>MSPILGYWKIKGLVQPTRLLLEYLEEKYEEHLYERDEGDKWRNKKFELGLEFPNLPYYIDGDVKLTQSMAIIRYIADKHNMLGGCPKERAEISMLEGAVLDIRYGVSRIAYSKDFETLKVDFLSKLPEMLKMFEDRLCHKTYLNGDHVTHPDFMLYDALDVVLYMDPMCLDAFPKLVCFKKRIEAIPQIDKYLKSSKYIAWPLQGWQATFGGGDHPPKSDLEVLFQGPLGSMALVPVGMAPRQMRVNRCIFASIVSFDACITYKSPCSPDAYHDDGWFICNNHLIKRFKMSKMVLPIFDEDDNQFKMTIARHLVGNKERGIKRILIPSATNYQDVFNLNSMMQAEQLIFHLIYNNENAVNTICDNLKYTEGFTSNTQRVIHSVYATTKSILDTTNPNTFCSRVSADELRFFDVTNARALRGGAGDQLFNNYSGFLQN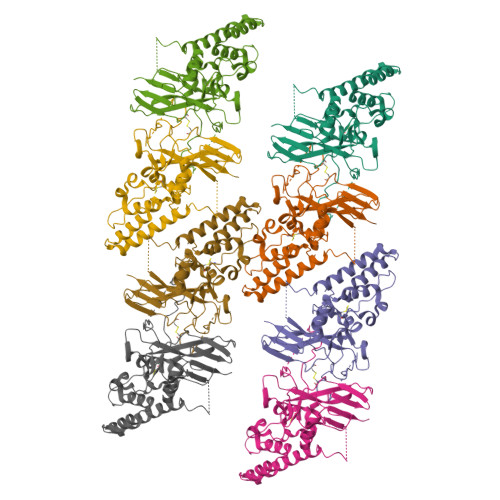LIRRAVAPEYLQIDTEELRFRNCATCIIDETGLVASVPDGPELYNPIRSSDIMRSQPNRLQIRNVLKFEGDTRELDRTLSGYEEYPTYVPLFLGYQIINSENNFLRNDFIPRANPNATLGGGAVAGPAPGVAGEAGGGIAVGGGGSGGGGSHHHHHHGGSGSSGGGGSSAHIVMVDAYKPTK[8x]>GPGSMTRKHIHFGVLIQGAGANMNAWKHPSVPPDASVNFDFYVDRARRAENAGIAFAFIADSAYVTPKSAPHFLNRFEPISLLSALAVLTSKIGLVGTMSSSYSEPYNVARQFASLDLISGGRAGWNVVTSSIEGTGKNYGRPHPDHAQRYAIAAEHLDVVQGLWDSWDDDALVRDRATGRFFDPDKLHRLDHRGRFFSVEGPLNIRRSPQGQPVIFQAGSSDDGIDLAGRSADAVFSNGSTFDEARVFYRRVKAAAAAAGRNPDH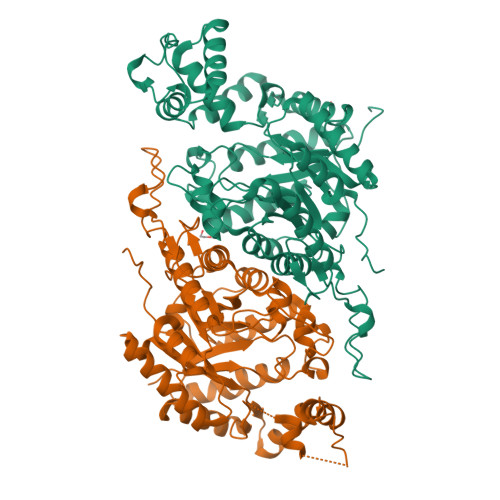VKVFPGIGPIVGATQQEADDKYRQVRDLLSPREALAYLSHFFQQHDFSVYPLDGPFPDIGTLGSDGFQSTTDNIKRLARERKLTLREVAYEVSTRRSNIGTSEAFIGTPEAVASEMIRWVDEGAADGFMLGLPVTGFGLDDFVDHVLPVLSARGYFDPVRRGATLRDHLGLPYKESRYARDAQVAAI[2x]> LK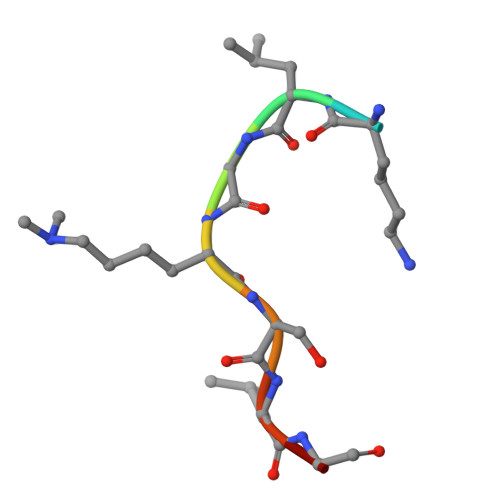LGKSLGR>HTDLSGKVFVFPRESVTDHVNLITPLEKPLQNFTLCFRAYSDLSRAYSLFSYNTQGRDNELLVYKERVGEYSLYIGRHKVTSKVIEKFPAPVHICVSWESSSGIAEFWINGTPLVKKGLRQGYFVEAQPKIVLGQEQDSYGGKFDRSQS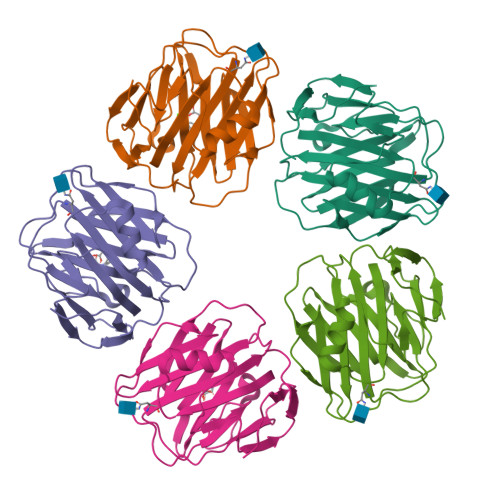FVGEIGDLYMWDSVLPPENILSAYQGTPLPANILDWQALNYEIRGYVIIKPLVWV[10x]>MGDTKEQRILRYVQQNAKPGDPQSVLEAIDTYCTQKEWAMNVGDAKGQIMDAVIREYSPSLVLELGAYCGYSAVRMARLLQPGARLLTMEINPDCAAITQQMLNFAGLQDKVTILNGASQDLIPQLKKKYDVDT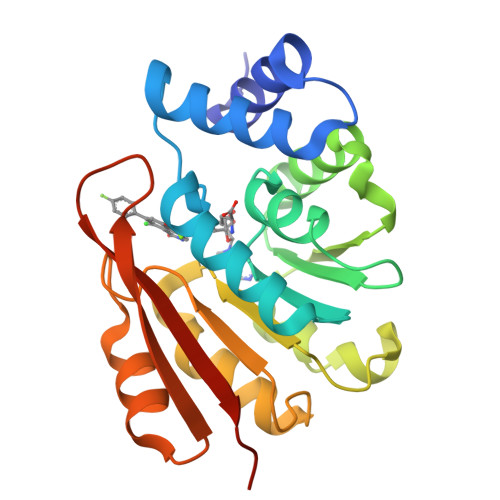LDMVFLDHWKDRYLPDTLLLEKCGLLRKGTVLLADNVIVPGTPDFLAYVRGSSSFECTHYSSYLEYMKVVDGLEKAIYQGPSSPDKS[2x]P. gingivalis is a heme auxotroph, therefore it must acquire this compound to survive and cause efficient infection establishment. Amongst well-characterized heme acquisition systems of P. gingivalis is that encoded by the hmu operon, comprising HmuR, a typical TonB-dependent receptor involved in heme transport across the outer membrane, HmuY, a heme-binding protein, and four proteins with unknown function. The work presented here substantially extends our knowledge of P. gingivalis HmuY by presenting data on further structural characterization of this protein and novel data on a second member of P. gingivalis HmuY-like family, Tfo produced by T. forsythia. The comparative analyses of HmuY homologs suggest that not only the HmuY hemophore-like protein of P. gingivalis, but also T. forsythia Tfo may be engaged in heme acquisition.

Our crystallographic studies have revealed a unique β-fold in the HmuY–heme protein structure and confirmed bis-histidine heme ligation. To further characterize P. gingivalis HmuY, we successfully solved its 3D structure in apo-form. Compared with holo-HmuY, one can see the opening up of the heme-binding pocket in the apo-form. The loop containing the axial heme ligand, His166, has moved significantly and the His166 side chain faces the surface of the apo-protein (the His166NE2 atom is shifted from the heme by approximately 16 Å). This loop must close up when the heme group enters the pocket. The opening up of the heme-binding pocket observed in the crystal structure of apo-protein was reproduced by MD. We experimentally verified that heme binding was accompanied by a movement of the loop carrying the His166 residue. Previously, using UV-visible spectroscopy with a single beam spectrophotometer, we estimated the Kd of heme binding under oxidizing conditions to the HmuY protein to be approximately 0.25 × 10−8 M. Here we carried out a more thorough analysis using a double-beam instrument and found that HmuY binds heme with Kd value < 10−9 M. We demonstrated that P. gingivalis HmuY not only binds free heme, but can wrest heme from methemoglobin directly and thus functions similar to typical secreted hemophores, which are engaged in heme transfer from the host hemoproteins to the outer membrane receptors.

>[2x]DEPNQPSTPEAVTKTVTIDASKYETWQYFSFSKGEVVNVTDYKNDLNWDMALHRYDVRLNCGESGKGKGGAVFSGKTEMDQATTVPTDGYTVDVLGRITVKYEMGPDGHQMEYEEQGFSEVITGKKNAQGFASGGWLEFSHGPAGPTYKLSKRVFFVRGADGNIAKVQFTDYQDAELKKGVITFTYTYPVK>[2x]MSINNEVQETLNKEVVQTKNSEYVQFESRSLLSLFTVGKIPPVDAAALCYWGEYDPEMFDWSRDYMIENIFENLPFWTMIKQTNWGRIAIIALPRFVSDLYSNQ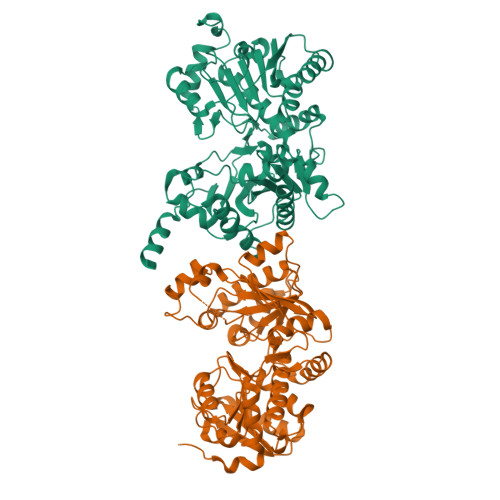DDAVQVIIEALEMAGIIGAKFVSLTGLIPSATDYGLAITKAVANREDLPKITTGHRTTGAAVVLTIKKICEQGGRDLSTEKVGFIGLGSVGMNVLPLMLKCLPHPQEITLCDVYSKLEFLENIEQNLVHKFGFKGKIKLALSKTTVPQEIYDSTLIVGATNVANVLDIMQVKPGTLIVDDSGPHCFSVEQAIKRFQEREDILFSEGGMLRSPFPIKTTVHLLPSVEKIMNNAQKEAVFNSNPFNIMGCAFSALLSSQFEQLEPTVGICDGEQSELHYQILQELEFEAGDLHCEHYVLPAKSIANFRQRFGKDLLEHHHHHH>MGNDISLIALLAFSTLLPFIIASGTCFVKFSIVFVMVRNALGLQQIPSNMTLNGVALLLSMFVMWPIMHDAYVYFEDEDVTFNDISSLSKHVDEGLDGYRDYLIKYSDRELVQFFENAQLKRQYGEETETVKRDKDEIEKPSIFALLPAYALSEIKSAFKIGFYLYLPFVVVDLVVSSVLLALGMMMMSPVTISTPIKLVLFVALDGWTLLSKGLILQYMDIAT[5x];> MFYALYFEIHHLVASAALGFARVAPIFFFLPFLNSGVLSGAPRNAIIILVALGVWPHALNEAPPFLSVAMIPLVLQEAAVGVMLGCLLSWPFWVMHALGCIIDNQRGATLSSSIDPANGIDTSEMANFLNMFAAVVYLQNGGLVTMVDVLNKSYQLCDPMNECTPSLPPLLTFINQVAQNALVLASPVVLVLLLSEVFLGLLSRFAPQMNAFAISLTVKSGIAVLIMLLYFSPVLPDNVLRLSFQATGLSSWFYERGATHVLE;>MDDLVFAGNKALYLVLILSGWPTIVATIIGLLVGLFQTVTQLQEQTLPFGIKLLGVCLCLFLLSGWYGEVLLSYGRQVIFLALAKG[4x];>[16x]MKTHILLARVLACAALVLVTPGYSSEKIPVTGSGFVAKDDSLRTFFDAMALQLKEPVIVSKMAARKKITGNFEFHDPNALLEKLSLQLGLIWYFDGQAIYIYDASEMRNAVVSLRNVSLNEFNNFLKRSGLYNKNYPLRGDNRKGTFYVSGPPVYVDMVVNAATMMDKQNDGIELGRQKIGVMRLNNTFVGDRTYNLRDQKMVIPGIATAIERLLQGEEQPLGNIVSSEPPAMPAFSANGEKGKAANYAGGMSLQEALKQNAAAGNIKIVAYPDTNSLLVKGTAEQVHFIEMLVKALDVAKRHVELSLWIVDLNKSDLERLGTSWSGSITIGDKLGVSLNQSSISTLDGSRFIAAVNALEEKKQATVVSRPVLLTQENVPAIFDNNRTFYTKLIGERNVALEHVTYGTMIRVLPRFSADGQIEMSLDIEDGNDKTPQSDTTTSVDALPEVGRTLISTIARVPHGKSLLVGGYTRDANTDTVQSIPFLGKLPLIGSLFRYSSKNKSNVVRVFMIEPKEIVDPLTPDASESVNNILKQSGAWSGDDKLQKWVRVYLDRGQEAIK;>[24x]MIRRYLYTFLLVMTLAGCKDKDLLKGLDQEQANEVIAVLQMHNIEANKIDSGKLGYSITVAEPDFTAAVYWIKTYQLPPRPRVEIAQMFPADSLVSSPRAEKARLYSAIEQRLEQSLQTMEGVLSARVHISYDIDAGENGRPPKPVHLSALAVYERGSPLAHQISDIKRFLKNSFADVDYDNISVVLSERSDAQLQAPGTPVKRNSFATSWIVLIILLSVMSAGFGVWYYKNHYARNKKGITADDKAKSSNE;>MSIATIVPENAVIGQAVNIRSMETDIVSLDDRLLQAFSGSAIATAVDKQTITNRIEDPNLVTDPKELAISQEMISDYNLYVSMVSTLTRKGVGAVETLLRS[6x];>[13x]MATPWSGYLDDVSAKFDTGVDNLQTQVTEALDKLAAKPSDPALLAAYQSKLSEYNLYRNAQSNTVKVFKDIDAAIIQNFR;>[24x]METSKEKTITSPGPYIVRLLNSSLNGCEFPLLTGRTLFVVGQSDALTASGQLPDIPADSFFIPLDHGGVNFEIQVDTDATEIILHELKEGNSESRSVQLNTPIQVGELLILIRPESEPWVPEQPEKLETSAKKNEPRFKNGIVAALAGFFILGIGTVGTLWILNSPQRQAAELDSLLGQEKERFQVLPGRDKMLYVAAQNERDTLWARQVLARGDYDKNARVINENEENKRISIWLDTYYPQLAYYRIHFDEPRKPVFWLSRQRNTMSKKELEVLSQKLRALMPYADSVNITLMDDVTAAGQAEAGLKQQALPYSRRNHKGGVTFVIQGALDDVEILRARQFVDSYYRTWGGRYVQFAIELKDDWLKGRSFQYGAEGYIKM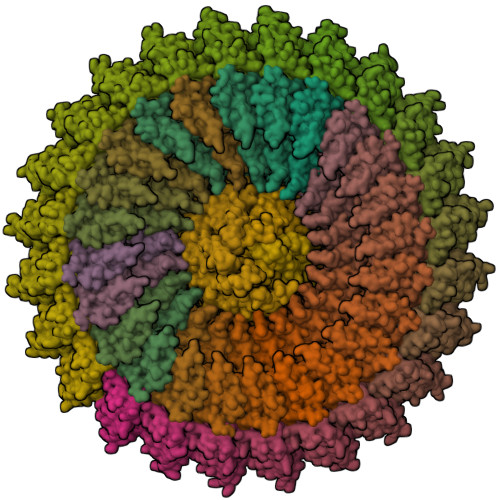SPGHWYFPSPL>[2x]RTNQAGLELIGNAEGCRRDPYMCPAGVWTDGIGNTHGVTPG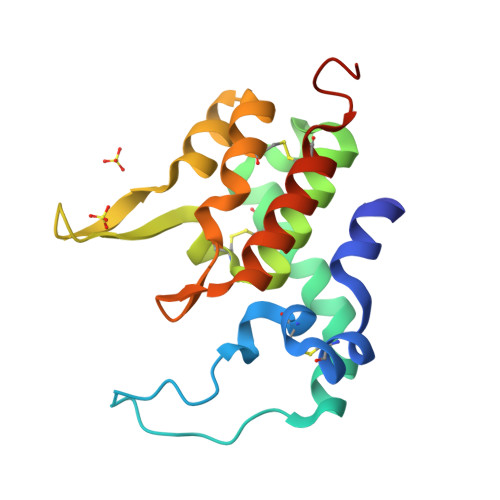VRKTDQQIAADWEKNILIAERCINQHFRGKDMPDNAFSAMTSAAFNMGCNSLRTYYSKARGMRVETSIHKWAQKGEWVNMCNHLPDFVNSNGVPLRGLKIRREKERQLCLTGLVNEHHHHHH> MGHHHHHHHHHHSSGHIEGRHMLRERTVRLQYGSRVEAVYVLGTYLWTDVYSAAPAGAQTFSLKHSEHVWVEVVRDGEAEEVATNGKQRWLLSPSTTLRVTMSQASTEASSDKVTVNYYDEEGSIPIDQAGLFLTAIEISLDVDADRDGVVEKNNPKKASWTWGPEGQGAILLVNCDRETPWLPKEDCRDEKVYSKEALKDMSQMILRTKGPDRLPAGYEIVLYISMSDSDKVGVFYVENPFFGQRYIHILGRRKLYHVVKYTGGSAELLFFVEGLCFPDEGFSGLVSIHVSLLEYMAQDIPLTPIFTDTVIFRIAPWIMTPNILPPVSVFVCCMKDNYLFLKEVKNLVEKTNCELKVCFQYLNRGDRWIQDEIEFGYIEAPHKGFPVVLDSPRDGNLKDFPVKELL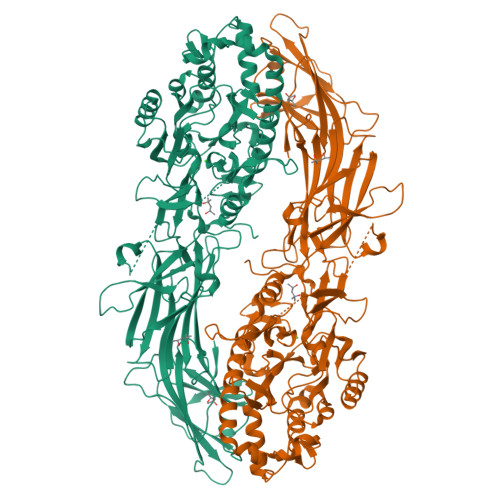GPDFGYVTREPLFESVTSLDSFGNLEVSPPVTVNGKTYPLGRILIGSSFPLSGGRRMTKVVRDFLKAQQVQAPVELYSDWLTVGHVDEFMSFVPIPGTKKFLLLMASTSACYKLFREKQKDGHGEAIMFKGLGGMSSKRITINKILSNESLVQENLYFQRCLDWNRDILKKELGLTEQDIIDLPALFKMDEDHRARAFFPNMVNMIVLDKDLGIPKPFGPQVEEECCLEMHVRGLLEPLGLECTFIDDISAYHKFLGEVHCGTNVRRKPFTFKWWHMVPSRRS>[2x]SKILVFGHQNPDSDAIGSSYAFAYLAREAYGLDTEAVALGEPNEETAFVLDYFGVAAPRVITSAKAEGAEQVILTDHNEFQQSVADIAEVEVYGVVDHHRVANFETANPLYMRLEPVGSASSIVYRMFKEHSVAVSKEIAGLMLSGLISDTLLLKSPTTHPTD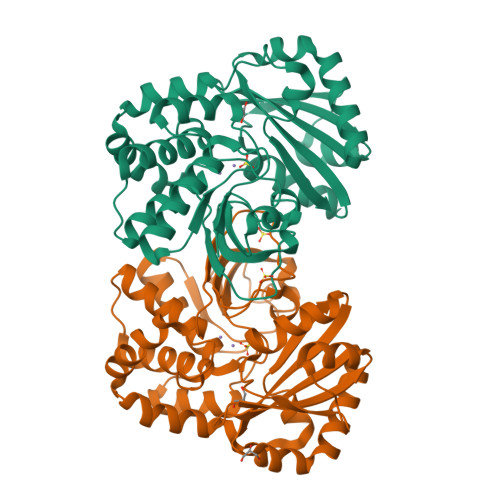KAIAPELAELAGVNLEEYGLAMLKAGTNLASKSAEELIDIDAKTFELNGNNVRVAQVNTVDIAEVLERQAEIEAAIEKAIADNGYSDFVLMITDIINSNSEILAIGSNMDKVEAAFNFVLENNHAFLAGAVSRKKQVVPQLTESFNA>[2x]MITIDGSYGEGGGQILRTSVALST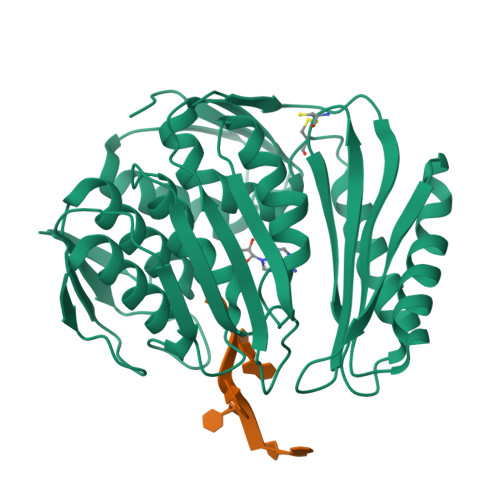ITGEPVRIVNIRANRPNPGLRPQHLHAILALKHLANAEVKGAHVGSRELVFIPKKLEAKEISIDIGTAGSITLVLQALLPAMVFAREKVKFRITGGTDVSWSPPVDYLSNVTLFALEKIGIHGEIRVIRRGHYPKGGGIVEGYVEPWNEKRELVAKEYSRIIKIEGISHATNLPSHVAERQARAAKDELLQLKVPIEIRTEISRSIGPGSGIVVWAETDCLRLGGDALGKKGKPAEIVGKEAAQELLDQLKPGHCVDKFLGDQLIPFLAFSGGVIWVSEITNHLKTNIWVVESFLGRIFDVDGNVGEPGKIRVIRRV>GPAVRTIRIYQPGEYQPGQLLELSPEAGQHVGVVLRMEQGEQLTLFNGDNKEFTASIERVKKKQVFVRIASVLEVNRESPLKIHLAQAISKGERMEMVMQKSAELGVACITPLITERCQVKIDKEKMAKKMHQWLNIIIGACEQCGRNQIPELRQPVYLDQFVRE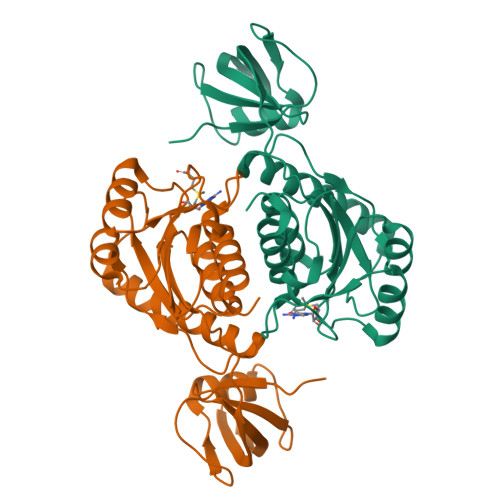AKEHLKLILHPAFSKTWRDYPVQPPDVALIIGPEGGFSDEEIRLTSGHGFLPLSLGPRVLRTETAAITALSVLQAAGGDL[8x]>[2x]GSELETDTREILEENNEMLHMYLNRLKTYQYLLKNEPIHVYYGSIDAYAEGIDKLLKTYADKMNLTASLCHYSTQADKDRLTEHMDDPADVQTRLDRK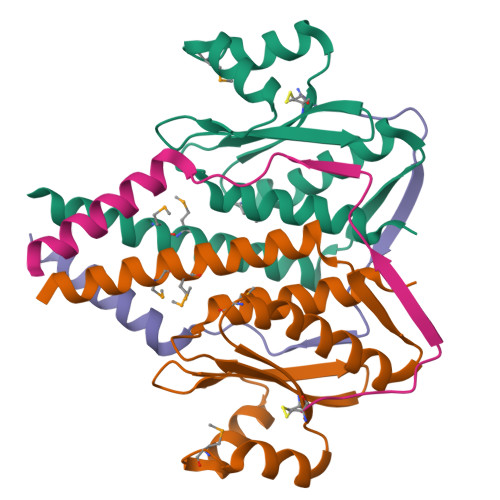DVYYDQYGKVVLIPFTIETQNYVIKLTSDSIVTEFDYLLFTSLTSIYDLVLPIEEEGEG;>[2x]MERAFQNRCEPRAAKPFKILKKRSTTSVASYQVSPHTARIFKENERLIDEYKRKKA> HHHHSSGLVPRGSHMAGHT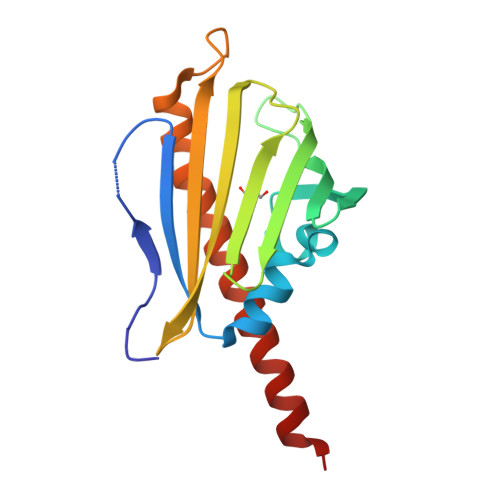DNEITIAAPMELVWNMTNDIEKWPGLFSEYASVEVLGRDDDKVTFRLTMHPDADGKVWSWVSERVADPVTRTVRAQRVETGPFQYMNIVWEYAETAEGTVMRWTQDFAMKPDAPVDDAWMTDNINRNSRTQMALIRDRIEQAAGERRTASVLAD> MDQECIENYAKVNGIYIYYKLCKAPEEKAKLMTMHGGPGM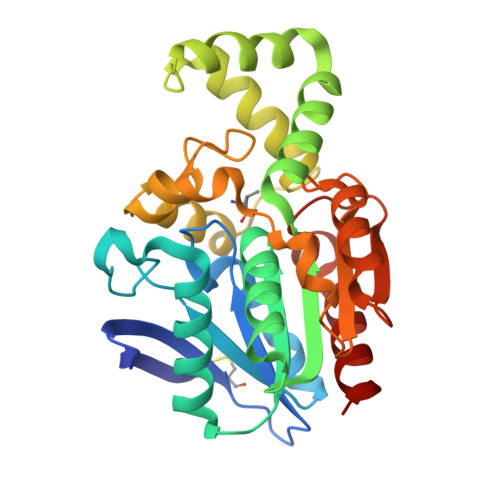SHDYLLSLRDMTKEGITVLFYDQFGCGRSEEPDQSKFTIDYGVEEAEALRSKLFGNEKVFLMGSSYGGALALAYAVKYQDHLKGLIVSGGLSSVPLTVKEMNRLIDELPAKYRDAIKKYGSSGSYENPEYQEAVNYFYHQHLLRSEDWPPEVLKSLEYAERRNVYRIMNGPNEFTITGTIKDWDITDKISAIKIPTLITVGEYDQVTPNVARVIHEKIAGSELHVFRDCSHLTMWEDREGYNKLLSDFILKHL>[2x]SMQPIVIHSSGKNYGFTIRAIRVYVGDSDIYTVHHIVWNVEEGSPACQAGLKA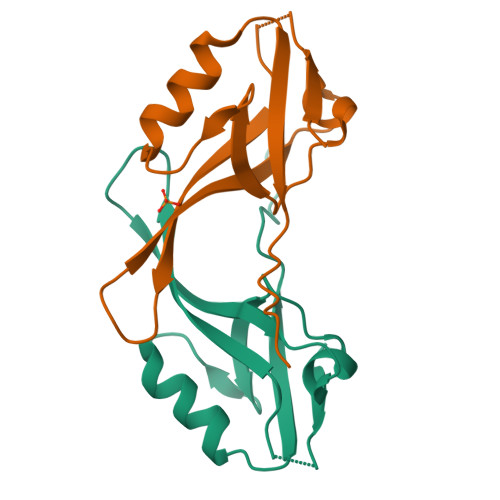GDLITHINGEPVHGLVHTEVIELLLKSGNKVSITTTPFENTETSV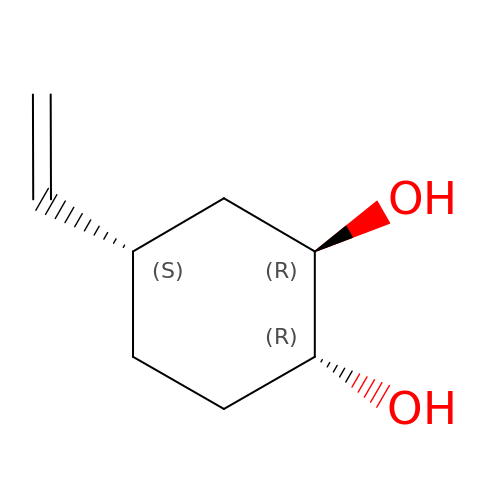(1R,2R,4S)-4-ethenylcyclohexane-1,2-diol | C8 H14 O2 | BSJHRRSHDADBTA-XLPZGREQSA-N4-(cyclopentylamino)-2-[(2-methoxybenzyl)amino]-N-[3-(2-oxopyrrolidin-1-yl)propyl]pyrimidine-5-carboxamide 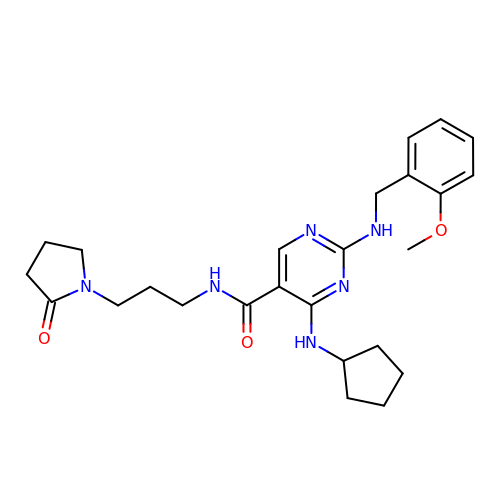| C25 H34 N6 O3 | ZXZLVQGNVOKCAS-UHFFFAOYSA-N>ANPLYQKHIISINDLSRDDLNLVLATAAKLKANPQPELLKHKVIASCFFEASTRTRLSFETSMHRLGASVVGFSDSANTSLGKKGETLADTISVISTYVDAIVMRHPQEGAARLATEFSGNVPV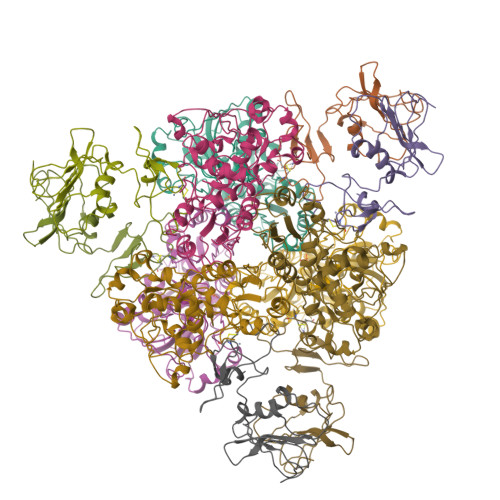LNAGDGSNQHPTQTLLDLFTIQETQGRLDNLHVAMVGDLKYGRTVHSLTQALAKFDGNRFYFIAPDALAMPQYILDMLDEKGIAWSLHSSIEEVMAEVDILYMTRVQKERLAPSEYANVKAQFVLRASDLHNAKANMKVLHPLPRVDEIATDVDKTPHAWYFQQAGNGIFARQALLALVLNRDLVL[2x];>[2x]MTHDNKLQVEAIKRGTVIDHIPAQIGFKLLSLFKLTETDQRITIGLNLPSGEMGRKDLIKIENTFLSEDQVDQLALYAPQATVNRIDNYEVVGKSRPSLPERIDNVLVCPNSNCISHAEPVSSSFAVRKRANDIALKCKYCEKEFSHNVVLAN> MKKIIYIATIGITLLTTSCDDFLDRQVPQGIVTGDQIASPEYVDNLVISAYAIWATGDDINSSFSLWNYDVRSDDCYKGGSGTEDGGVFNALEISKGINTTDWNINDIWKRLYQCITRANTALQSLDQMDEKTYPLKNQRIAEMRFLRGHAHFMLKQLFKKIVIVNDENMEPDAYNELSNTTYTNDEQWQKIA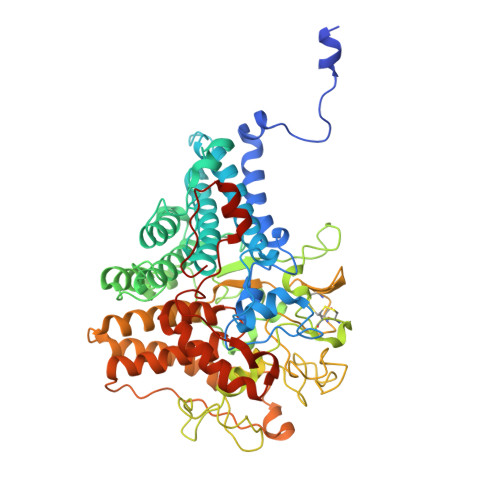DDFQFAYDNLPEVQIEKGRPAQAAAAAYLAKTYLYKAYRQDGADNALTGINEEDLKQVVKYTDPLIMAKGGYGLETDYSMNFLPQYENGAESVWAIQYSINDGTYNGNLNWGMGLTTPQILGCCDFHKPSQNLVNAFKTDSQGKPLFSTYDNENYEVATDNVDPRLFHTVGMPGFPYKYNEGYIIQKNDDWSRSKGLYGYYVSLKENVDPDCDCLKKGSYWASSLNHIVIRYADVLLMRAEALIQLNDGRITDAISLINEVRSRAAGSTMLIFNYKEDYGVNFKVTPYDLKAYAQDEAMKMLKWERRVEFGMESSRFFDLVRWGEAKDVINAYYVTEASRCSIYKNAGFTENKNEYLPVPFEQISASNGNYTQNFGWHHHHHH>MKKIAIFAGDGIGPEIVAAARQVLDAVDQAAHLGLRCTEGLVGGAALDASDDPLPAASLQLAMAADAVILGAVGGPRWDAYPPAKRPEQGLLRLRKGLDLYANLRPAQIFPQLLDASPLRPELVRDVDILVVRELTGDIYFGQPRGLEVIDGKRRGFNTMVYDEDEIRRIAHVAFRAAQGRRKQLCSVDKANVLETTRLWREVVTEVARDYPDVRLSHMYVDNAAMQLIRAPAQFDVLLTGNMFGDILSDEASQLTGSIGMLPSASLGEGRAMYEP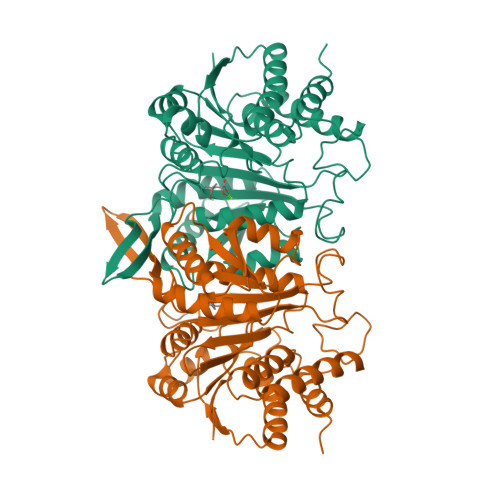IHGSAPDIAGQDKANPLATILSVAMMLRHSLNAEPWAQRVEAAVQRVLDQGLRTADIAAPGTPVIGTKAMGAAVVNALNLKD[2x]>[4x]MSQHNEKNPHQHQSPLHDSSEAKPGMDSLAPEDGSHRPAAEPTPPGAQPTAPGSLKAPDTRNEKLNSLEDVRKGSENYALTTNQGVRIADDQNSLRAGSRGPTLLEDFILREKITHFDHERIPERIVHARGSAAHGYFQPYKSLSDITKADFLSDPNKITPVFVRFSTVQGGAGSADTVRAIRGFATKFYTEEGIFDLVGNNTPIFFIQDAHKFPDFVHAVKPEPHWAIPQGQSAHDTFWDYVSLQPETLHNVMWAMSDRGIPRSYRTMEGFGIHTFRLINAEGKATFVRF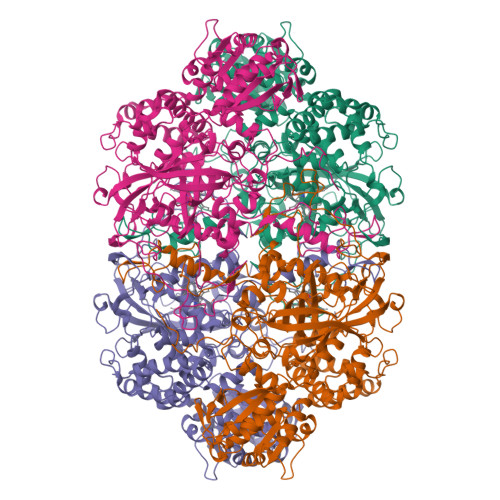HWKPLAGKASLVWDEAQKLTGRDPDFHRRELWEAIEAGDFPEYELGFQLIPEEDEFKFDFDLLDPTKLIPEELVPVQRVGKMVLNRNPDNFFAENEQAAFHPGHIVPGLDFTNDPLLQGRLFSYTDTQISRLGGPNFHEIPINRPTCPYHNFQRDGMHRMGIDTNPANYEPNSINDNWPRETPPGPKRGGFESYQERVEGNKVRERSPSFGEYYSHPRLFWLSQTPFEQRHIVDGFSFELSKVVRPYIRERVVDQLAHIDLTLAQAVAKNLGIELTDDQLNITPPPDVNGLKKDPSLSLYAIPDGDVKGRVVAILLNDEVRSADLLAILKALKAKGVHAKLLYSRMGEVTADDGTVLPIAATFAGAPSLTVDAVIVPCGNIADIADNGDANYYLMEAYKHLKPIALAGDARKFKATIKIADQGEEGIVEADSADGSFMDELLTLMAAHRVWSRIPKIDKIPA In M. capsulatus (Bath), two related β-sheet proteins (31% sequence identity) have been previously identified, a cytochrome P460 (McP460) and a cytochrome c′ (McCP-β)5,6 encoded by the CytL and CytS genes respectively. Cytochromes P460, defined by an unusual porphyrin-Lys cross link at the 13′ meso carbon, catalyse the oxidation of hydroxylamine (NH2OH) to form N2O under anaerobic conditions. In contrast, cyts cp-β (the only known cytochromes c′ with a β-sheet fold) lack this crosslink and appears to be optimized for binding non-polar molecules (including NO and CO) without enzymatic conversion. High resolution crystal structures reveal a highly similar tertiary structure between the two proteins but major structural differences around the heme pocket consistent with a switch of function between hydroxylamine oxidation (P460) and NO binding/sequestration (cyt cp-β).

The crystal structure of as-isolated (ferric) McP460 was determined to 1.36 Å resolution with residues 19 to 161 observed in the electron density maps. McP460 exists as a homodimer, with each monomer consisting of a twisted five-stranded antiparallel β-sheet, two α-helices and two helical turns, Fig. 1A – a protein fold similar to that of NeP460 12 and NsALP460 13 from AOB. The defining P460 covalent cross-link is evident between Lys 78 and the 13′-meso carbon of the McP460 porphyrin ring. No hydroxyl modification of the porphyrin (observed at the 5′-meso carbon position in NeP460, but not in NsALP460) is evident in our McP460 structure. The proximal pocket of McP460 is also quite similar to that of NeP460 and NsALP460, a minor difference being that the His 144 ligand of McP460 is H-bonded to the Tyr 119 peptide carbonyl, whereas the His ligands of NeP460 and NsALP460 are H-bonded to a Met carbonyl. The distal water ligand in McP460 is 3.1/3.2 Å from residue Asp 102, and we note that a bound hydroxylamine substrate displacing the distal water would likely be in hydrogen-bonding distance to several additional pocket residues such as Arg 43, Arg 50, Asp 102 or Arg 121. By contrast, our structure of McP460 clearly shows a 6c Fe(iii) heme resting state, similar to that of the HAO P460 cofactor. McP460 has a significantly more hydrophilic pocket, which may allow water ingress and aid in denaturation.

>MRKLAIALLFPAAAVLAEPAAAPNGISLPAGYKDWKMIGVSSRIEQNNLRAILGNDIAVKAAREGRTHPWPDGAILVKLSWKKSTHELFPSAEVPGDFTQADFMVKDAAKYASTGGWGYARWLGMEQKPYGANADFAQECMGCHSGAKAADYVFTHPAKLP[2x]>MEDLNFRKGDAKTDVFGSDRMLQPSPVERIPDGPTTPEVAYQMVKDETFAQTQPRLNLATFVTTYMDDYATKLMNEAININYIDETEYPRIAVMNGKCINIVANLWNSPEKDTWKTGALAIGSSEACMLGGVAAWLRWRKKRQAQGKPFDKPNFVISTGFQVVWEKFAQLWQIEMREVPLTLEKTTLDPEEALKMCDENTICVVPIQGVTWTGLNDDVEALDKALDAYNAKTGYDIPIHVDAASGGFILPFLYPDTKWDFRLKWVLSISVSGHKFG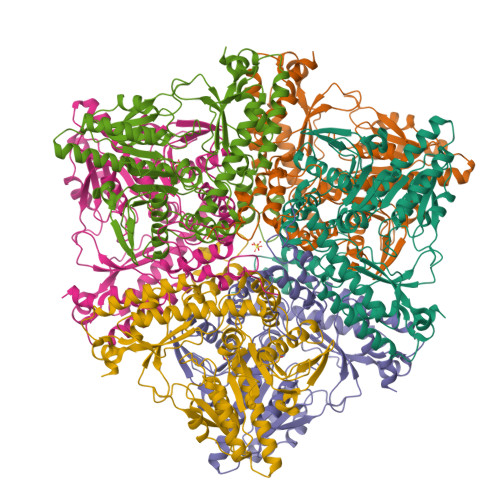LVYPGLGWVCWKGKEYLPEEMSFSVNYLGANITQVGLNFSRPAAQILGQYYQFIRLGFQGYKEVQYNSLQIAKYIHGEIAKMAPFVNYSENVVNPLFIWYLKPEYAKSAKWTLYDLQDKLSQHGWMVPAYTLPSKLEDYVVMRVVVRQGFSRDMADMLLGDIKNAIAELEKLDFPTPTRMAQEKNLPVEAKMFNHGGRRHKTVKK[6x]>[4x]GDELLNICMNAKHHKRVPSPEDKLYEECIPWKDNACCTLTTSWEAHLDVSPLYNFSLFHCGLLMPGCRKHFIQAICFYECSPNLGPWIQPVGSLGWEVAPSGQGERVVNVPLCQEDC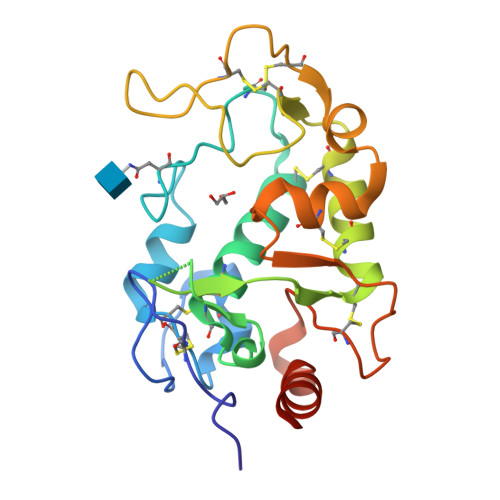EEWWEDCRMSYTCKSNWRGGWDWSQGKNRCPKGAQCLPFSHYFPTPADLCEKTWSNSFKASPERRNSGRCLQKWFEPAQGNPNVAVARLFASGRLVPR>GSHMSELEKAMVALIDVFHQYSGREGDKHKLKKSELKELINNELSHFLEEIKEQEVVDKVMETLDNDGDGECDFQEFMAFVAM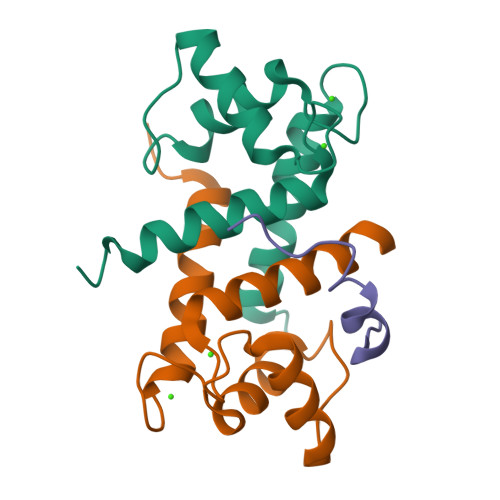VTTACHEFFEHE[2x];> GSQSQLSHQDLQLVKGAMAATYSALNSSKPTPQLKPIESS> MVAPKPKPAHEQVEPALIPSNWTSVIPLLTSDFKNQYSVISRLKNPNMKPVPYAGDIIKLMAFINKFSSFFHSDLQNLSFQDFEVGLDLYPGDPNGSAAGIVKGPEDTSLLLYPDFMAIKDIVYCQDKMNLLFLSLLDLTFTENFDGKSAKKKGPLTTWENLKSSSKKVFSNPLYRLRLVAREWGYPREWRQQLPSDQDISKPKTALFEQDEQTPVVDPSHPEILTPNIYTWNANEPLPLESNPLYNREMDKNGILALKPMDRVVLLRALTDWCASHSSAIHDEIYKLTHGKKDPVFGIQTQQVPRYTIEGVDNTINQFKKLCSLIQSRYEIRSKKKHFVKQLKEGKKPDLSRKLEILKEIKAELKNAVKSEKDELLFSLYDKWVPLFEGELPDQPLANPFSERLYKLRLQEFFLGRVPHIGDFYMPRLHSYGDSLEMSTFTDLRNLQALLSKFKNNEYNAFTLFENDGQSMSAQFKLFYHDTPSLAHDVARGRNTSGKVYWYELCHDSATLLEFLEFLDYKIVKPQDEKKEGNEKEKEALNNEAHILEQKSTTDNKPSINTNPLPKDAKYNTARKKLQILKEFLSDYYFILRQFEQMKVQFADMKPGKRQ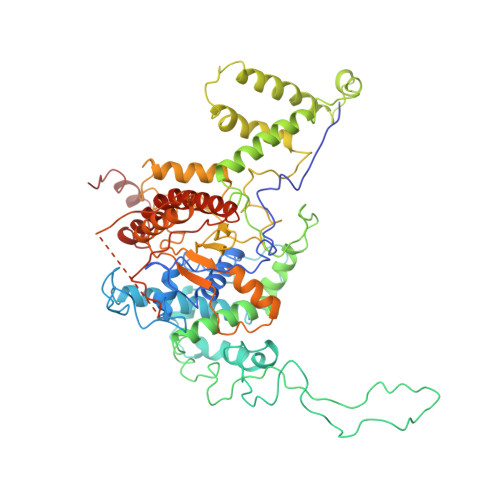LRRIQRQTVNYNT>KPFKCSMCDYASVEVSKLKRHIRSHTGERPFQCSLCSYASR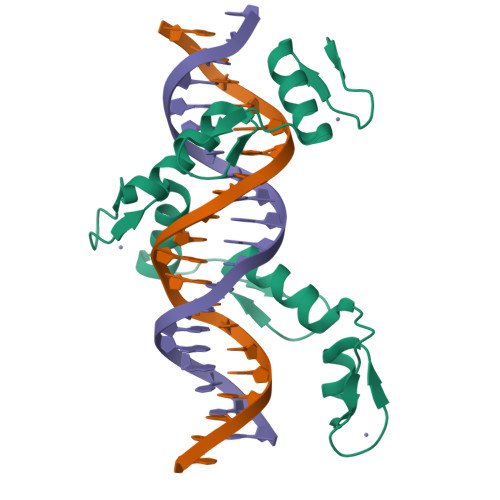DTYKLKRHMRTHSGEKPYECYICHARFTQSGTMKMHILQKHTENVAKFHCPHCDTVIARKSDLGVHLRKQHSYIEQGKKCRYCDAVFHERYALIQHQKSHK[2x]>[1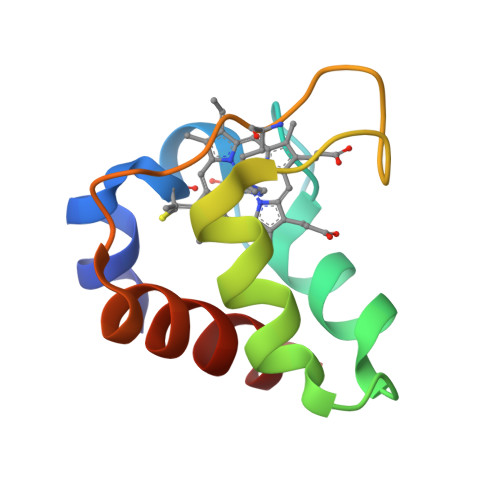8x]DADLAKKNNCIACHQVETKVVGPALKDIAAKYADKDDAATYLAGKIKGGSSGVWGQIPMPPNVNVSDADAKALADWILTLK Sin is a resolvase of the serine recombinase family that is encoded by various S. aureus multiresistance plasmids (Paulsen et al., 1994; Rowland and Dyke, 1989). It is thought to stabilize plasmids by resolving dimers into monomers. Each res site binds two dimers of Sin, at sites I and II, and a nonspecific DNA-bending protein, e.g., HU (Rowland et al., 2002). Synapsis of the regulatory Sin dimers at site II is thought to initiate assembly of the synaptic complex, leading to formation of an active catalytic tetramer at site I (Rowland et al., 2002).

To address these issues, we have solved the crystal structure of a wild-type (WT) Sin dimer bound to a site II duplex. WT Sin was cocrystallized with a 29 bp DNA duplex containing the site II direct repeat (Rowland et al., 2002). Each Sin monomer is composed of a mixed αβ N-terminal catalytic domain and a helix-turn-helix (HTH) CTD that are linked through an extended helix (helix E), which forms the majority of the dimerization interface. The site II-bound Sin dimer is markedly asymmetric, reflecting the requirement for the CTDs to dock with DNA repeat motifs in a head-to-tail configuration. However, in the Sin-site II complex, the bends in helix E are more drastic and asymmetric than those seen in γδ-site I complexes and only one E helix is inserted into the minor groove. Sin bound to site II is catalytically inactive. The catalytic serines are >12 Å from the DNA and are partially blocked from it by the E helix of the other monomer. The second potential tetramer interface buries substantially more surface area (1865 Å2) and is composed entirely of contacts between the DNA-binding domains (CTDs), primarily the N-terminal portions of each helix F. The Sin tetramer defined by this interface places the binding domains and associated DNA duplexes near the center of the complex with the catalytic domains on the outside. The duplexes cross each other at a ∼60° angle to form a negative node and are <10 Å apart.

>MIIGYARVSSLDQNLERQLENLKTFGAEKIFTEKQSGKSIENRPILQKALNFVRMGDRFIVESIDRLGRNYNEVIHTVNYLKDKEVQLMITSLPMMNEVIGNPLLDKFMKDLIIQILAMVSEQERNESKRRQAQGIQVAKEKGVYKGRPLLYSPNAKDPQKRVIYHRVVEMLEEGQAISKIAKEVNITRQTVYRIKHDNGLSSHHHHHH[4x]The α-amylase from the psychrophilic bacterium Pseudoalteromonas haloplanktis (AHA) is probably the most thoroughly studied cold-adapted enzyme that shows such an anomalous T-optimum, which, in this case, is about 15°C lower than the melting temperature (Tm). Earlier computer simulations of the catalytic reactions of AHA and PPA, based on molecular dynamics (MD) free energy calculations using the empirical valence bond (EVB) method, could directly reproduce the T-optimum of AHA and explain its origin. It was found that a particular binding interaction, between Asp264 of the enzyme and the 2′- and 3′-hydroxyl groups at the −1 position of the oligosaccharide substrate, starts to break precisely at room temperature. Since only the cold-adapted AHA enzyme showed instability of the Asp264-substrate interaction above room temperature, we hypothesized that if its β7-α7 loop conformation could be brought to that found in PPA, then its T-optimum could possibly be raised. In particular, the final model (Chimera 4) that combines 16 mutations in all of the four identified regions above is predicted to almost entirely recover the stable hydrogen bond interaction between Asp264 and the substrate at 25°C, as opposed to the wild-type (WT) enzyme.

To structurally evaluate our computational design, we determined the crystal structures of Chimera 4 in its apo form and in complex with the inhibitor acarbose. The inhibitor is known to be rearranged by α-amylases in crystal soaking experiments to form several different products. The variant observed in the active site here was a pseudo-pentasaccharide which has also been observed in human PPA. As can be seen in Fig. 5A, the mutated side chains in Chimera 4 are all very close to their position in the corresponding complex with mesophilic PPA. The only exception is the NDW motif (residues 311 to 313) where the side-chain conformations differ somewhat. It appears that the extended β2-α2 and β8-α8 loops in PPA that pack against this motif are responsible for these differences, as Chimera 4 retains the shorter loops from AHA. The electron density is weak for the two residues Ala271 and Gly272 of the remodeled β7-α7 loop, in both the apo- and holo-structures, so that their backbone conformation cannot be confidently built. There is, however, clear indication from the partial density that the loop conformation is closer to that of PPA than AHA, as intended for Chimera 4. The mobility of the β7-α7 loop in the Chimera 4 complex with acarbose, as well as in PPA, is considerably less flexible than in AHA.

> HPTTFVHLFEWNWQDVAQECEQYLGPKGYAAVQVSPPNEHITGSQWWTRYQPVSYELQSRGGNRAQFIDMVNRCSAVGVDIYVDTLINHMAAGSGTGTAGNSFGNKSFPIYSPQDFHESCTINNSDYGNDRYRVQNCELVGLADLDTASNYVQNTIAAYINDLQAIGVKGFRFDASKHVAASDIQSLMAKVNGSPVVFQEVIDLGGEAIKSSEYLSTGLVTEFKYGAKLGTVFRNGSLAWLSNFGEGWGFMPSSSAVVFVDNHDNQRGHGAGGSSILTFEDGRLYDLANVFMLAYPYGYPRVMSSYDFHGNDWAGGPNVPVHNNGNLECFASNWKCEHRWSYIAGGVDFRNNTADNWAVTNWWDNTNNQISFGRGSSGHMAINKEDSTLTATVQTDMASGQYCNVLKGELSADAKSCSGEVITVNSDGTINLNIGAWDAMAIHKNAKLGA>[8x]GSQIHVDTMKVINDPIHGHIELHPLLVRIIDTPQFQRLRYIKQLGGGYYVFPGASHNRFEHSLGVGYLAGCLVHALGEKQPELQISERDVLCVQIAGLCHDLGHGPFSAMFDGRFIPLARPEVKWTHEQGSVMMFEHLINSNGIKPVMEQYGLIPEEDICFIKEQIVGPLESPVEDSLWPYKGRPENKSFLYEIVSNKRNGIDVDKWDYFARDCHHLGIQNNFDYKRFIKFARVCEVDNELRICARDKEVGNLYDMFHTRNSLHRRAYQHKVGNIIDTMITDAFLKADDYIEITGAGGKKYRISTAIDDMEAYTKLTDNIFLEILYSTDPKLKDAREILKQIEYRNLFKYVGETQPTGQIKIKREDYESLPKEVASAKPKVLLDVKLKAEDFIVDVINMDYGMQEKNPIDHVSFYCKTAPNRAIRITKNQVSQLLPEKFAEQLIRVYCKKVDRKSLYAARQYFVQWCADRNFTKPQDGDVIAPLITPQKKEWNDSTSVQNPTRLREASKSRVQLFKDDPM

Sterile alpha motif and HD domain-containing protein 1 (SAMHD1) is an important regulator of cellular 2′-deoxynucleoside-5′-triphosphate (dNTP) in mammalian cells. Although the HD-domain contains the active site, dNTP hydrolysis requires assembly of SAMHD1 into homo-tetramers. Here, sequences at the N and C termini of the HD-domain stabilise inter-monomer protein–protein interactions and incorporate four pairs of allosteric nucleotide-binding sites, AL1 and AL2, which regulate the enzyme through combined binding of G-based (AL1) and 2′-deoxynucleoside (AL2) triphosphates. Using combined biophysical and X-ray structural studies incorporating nucleotide analogues along with mutagenesis experiments we have now discovered that SAMHD1 uses a bi-metallic Fe–Mg centre to catalyse dNTP hydrolysis in a reaction similar to those catalysed by HD domains in both human and bacterial phosphodiesterase PDE enzymes.

In our proposed mechanism, His215 is the general acid that stabilises evolving negative charge at the O5′ during the ES to EP transition and likely protonates the O5′ on the 2′-deoxynucleoside leaving group. However, no measurable triphosphohydrolase activity could be detected for the H215A mutant, even when elevated levels (10 µM) of H215A–SAMHD1 were employed in the assay, confirming its critical function in catalysis. In the structure, the bound active site dAMPNPP nucleotide adopts the same configuration as that observed in the wt and D137N structures. A 3D structural superimposition of the H215A and wt structures based on alignment of all SAMHD1 atoms reveals an overall rmsd of only 0.531 Å. In addition, the active site side chains, metal ions and water molecule positions are also maintained in the same positions as in the wt active site further supporting His215 function in catalysis at a stage subsequent to tetramer formation and binding of the substrate. In addition, we solved a further structure of the catalytically inactive mutant H215A, which does not disrupt metal ion binding, with dAMPNPP bound in the active site. In all our structures the active site side chain configurations, nucleotide conformation and metal ion–water network are all conserved, including in the H215A structure. These observations support the notion that, although critical for catalysis, His215 is not required for substrate binding.> MATPDQKSPNVLLQNLCCRILGRSEADVAQQFQYAVRVIGSNFAPTVERDEFLVAEKIKKELIRQRREADAALFSELHRKLHSQGVLKNKWSILYLLLSLSEDPRRQPSKVSSYATLFAQALPRDAHSTPYYYARPQTLPLSYQDRSAQSAQSSGSVGSSGISSIGLCALSGPAPAPQSLLPGQSNQAPGVGDCLRQQLGSRLAWTLTANQPSSQATTSKGVPSAVSRNMTRSRREGDTGGTMEITEAALVRDILYVFQGIDGKNIKMNNTENCYKVEGKANLSRSLRDTAVRLSELGWLHNKIRRYTDQRSLDRSFGLVGQSFCAALHQELREYYRLLSVLHSQLQLEDDQGVNLGLESSLTLRRLLVWTYDPKIRLKTLAALVDHCQGRKGGELASAVHAYTKTGDPYMRSLVQHILSLVSHPVLSFLYRWIYDGELEDTYHEFFVASDPTVKTDRLWHDKYTLRKSMIPSFMTMDQSRKVLLIGKSINFLHQVCHDQTPTTKMIAVTKSAESPQDAADLFTDLENAFQGKIDAAYFETSKYLLDVLNKKYSLLDHMQAMRRYLLLGQGDFIRHLMDLLKPELVRPATTLYQHNLTGILETAVRATNAQFDSPEILRRLDVRLLEVSPGDTGWDVFSLDYHVDGPIATVFTRECMSHYLRVFNFLWRAKRMEYILTDIRKGHMCNAKLLRNMPEFSGVLHQCHILASEMVHFIHQMQYYITFEVLECSWDELWNKVQQAQDLDHIIAAHEVFLDTIISRCLLDSDSRALLNQLRAVFDQIIELQNAQDAIYRAALEELQRRLQFEEKKKQREIEGQWGVTAAEEEEENKRIGEFKESIPKMCSQLRILTHFYQGIVQQFLVLLTTSSDESLRFLSFRLDFNEHYKAREPRLRVSLGTRGRR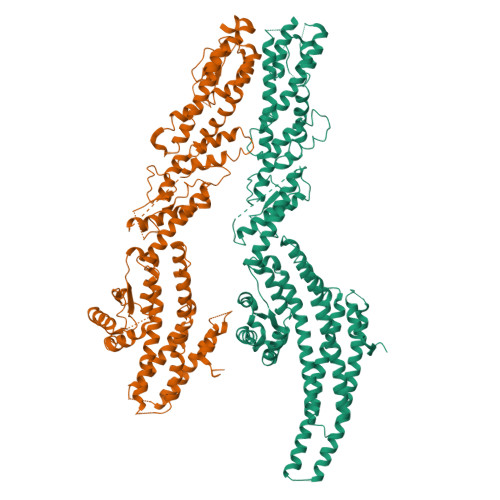SSHT;> MSEFRIHHDVNELLSLLRVHGGDGAEVYIDLLQKNRTPYVTTTVSAHSAKVKIAEFSRTPEDFLKKYDELKSKNTRNLDPLVYLLSKLTEDKETLQYLQQNAKERAELAAAAVGSSTTSINVPAAASKISMQELEELRKQLGSVATGSTLQQSLELKRKMLRDKQNKKNSGQHLPIFPAWVYERPALIGDFLIGAGISTDTALPIVLLRWNLALSPRLKCSGVISAHCNLHLPGTLPLASQESAVVEDLLYVLVGVDGRYVSAQPLAGRQSRTFLVDPNLDLSIRELVHRILPVAASYSAVTRFIEEKSSFEYGQVNHALAAAMRTLVKEHLILVSQLEQLHRQGLLSLQKLWFYIQPAMRTMDILASLATSVDKGECLGGSTLSLLHDRSFSYTGDSQAQELCLYLTKAASAPYFEVLEKWIYRGIIHDPYSEFMVEEHELRKERIQEDYNDKYWDQRYTIVQQQIPSFLQKMADKILSTGKYLNVVRECGHDVTCPVAKEIIYTLKERAYVEQIEKAFNYASKVLLDFLMEEKELVAHLRSIKRYFLMDQGDFFVHFMDLAEEELRKPVEDITPPRLEALLELALRMSTANTDPFKDDLKIDLMPHDLITQLLRVLAIETKQEKAMAHADPTELALSGLEAFSFDYIVKWPLSLIINRKALTRYQMLFRHMFYCKHVERQLCSVWISNKTAKQHSLHSAQWFAGAFTLRQRMLNFVQNIQYYMMFEVMEPTWHILEKNLKSASNIDDVLGHHTGFLDTCLKDCMLTNPELLKVFSKLMSVCVMFTNCMQKFTQSMKLDGELGGQTLEHSTVLGLPAGAEERARKELARKHLAEHADTVQLVSGFEATINKFDKNFSAHLLDLLARLSIYSTSDCEHGMASVISRLDFNGFYTERLERLSAERSQKATPQVPVLRGPPAPAPRVAVTAQ> MAYVLDTNVAIHLRDGDPEVTTRVTALNGAILLSIISRVELEGGVYREAAQAGLRRSRLDVMLKVLPVLDFDGAAADEYRRIVESAGYSRRK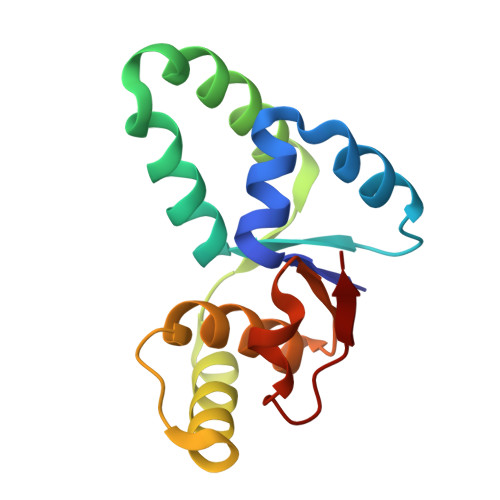VVDRMIAAQALAHRATFVTFNADDFRDIPGLSLLAW>ADPLLLYANRRDLRLVDATNGKENATIVVGGLEDAAAVDFVFSHGLIYWSDVSEEAIKRTEFNKTESVQNVVVSGLLSPDGLACDWLGEKLYWTDSETNRIEVSNLDGSLRKVLFWQELDQPRAIALDPSSGFMYWTDWGEVPKIERAGMDGSSRFIIINSEIYWPNGLTLDYEEQKLYWADAKLNFIHKSNLDGTNRQAVVKGSLPHPFALTLFEDILYWTDWSTHSILACNKYTGEGLREIHSDIFSPMDIHAFSQQRQPNATNPCGIDNGGCSHLCLMSPVKPFYQCACPTGVKLLENGKTCKDGATELLLLARRTDLRRISLDTPDFTDIVLQLEDIRHAIAIDYDPVEGYIYWTDDEVRAIRRSFIDGSGSQFVVTAQIAHPDGIAVDWVARNLYWTDTGTDRIEVTRLNGTMRKILISEDLEEPRA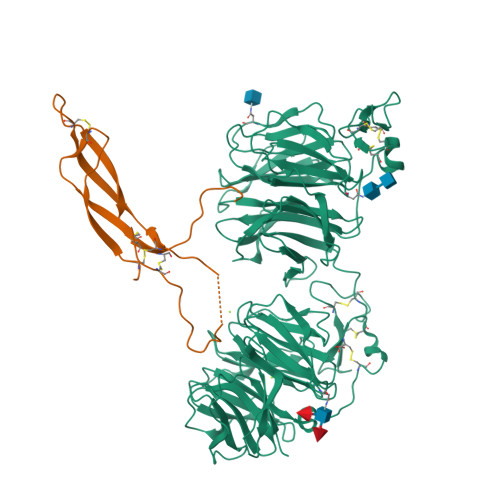IVLDPMVGYMYWTDWGEIPKIERAALDGSDRVVLVNTSLGWPNGLALDYDEGKIYWGDAKTDKIEVMNTDGTGRRVLVEDKIPHIFGFTLLGDYVYWTDWQRRSIERVHKRSAEREVIIDQLPDLMGLKATNVHRVIGSNPCAEENGGCSHLCLYRPQGLRCACPIGFELISDMKTCIVPHHHHHHHHHH[2x];>[2x]GPSRQGWQAFKNDATEIIPELGEYPEPPPELENNKTMNRAENGGRPPHHPFETKDVSEYSCRELHFTRYVTDGPCRSAKPVTELVCSGQCGPARLLPNAIGRGKWWRPSGPDFRCIPDRYRAQRVQLLCPGGEAPRARKVRLVASCKCKRLTRFHNQS> GSMRHERVVIIKNMFHPMDFEDDPLVLNEIREDLRVECSKFGQIRK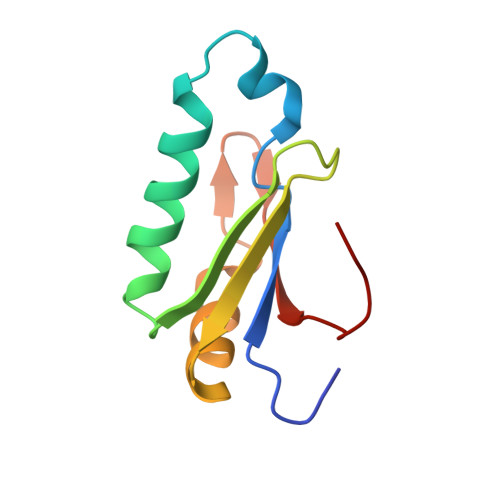LLLFDRHPDGVASVSFRDPEEADYCIQTLDGRWFGGRQITAQAWDGTTDY The tripartite motif (TRIM) proteins form one of the largest subfamilies of RING-type E3 ubiquitin ligases, comprising more than 80 members. TRIM family members typically contain a RING domain usually catalyzing ubiquitin transfer; one or two B-box domains mediating protein–protein interactions; and a large coiled-coil domain region, which is involved in self-association or oligomerization with other TRIM E3-ligase proteins (Fiorentini et al., 2020, Ozato et al., 2008). About two-thirds of human TRIM proteins feature a PRYSPRY domain, also known as the B30.2 domain, in their C-terminal region. All characterized family members shared the same overall PRYSPRY twisted β-sandwich fold consisting of a 7-stranded and a 6-stranded antiparallel β-sheet.

Conversely, the TRIM36 PRYSPRY domain has characteristic loop insertions, which also affects its oligomerization state. The crystal lattice of the TRIM36 PRYSPRY domain contained four molecules in the asymmetric unit, forming two essentially identical symmetrical dimers. This observation is consistent with the TRIM36 domain eluting in gel filtration with a Superdex-75 column at a retention time corresponding to a dimer. The dimer interface is formed by a helix-turn-strand insertion between the canonical β-strands 2 and 3 of the PRY subdomain. The additional β-strand, β2′, self-assembled into a two-stranded antiparallel intermolecular β-sheet, and Phe543, Leu545, Leu547, and Ile552, located on the helix, form hydrophobic packing interactions with the adjacent monomer. The total dimer interface area is 1803 Å2 for chains A and B, and 1875 Å2 for chains C and D. The same PRYSPRY dimer interface was also predicted in the AlphaFold3 model of the full-length protein of TRIM36, and the related TRIM46 homolog, in addition to the typical dimerization via the coiled-coil domain. An unusually large insertion was observed between the canonical β-strands 5 and 6, featuring an additional helix and a long disordered segment. Another noteworthy feature of the TRIM36 structure is a unique helical extension at the C-terminus. A systematic analysis of this canonical substrate-binding region in the PRYSPRY structures determined in this study revealed significant variations and distinct surface properties across different family members, providing intriguing insights into the divergent evolution of TRIM family members. This canonical binding site was accessible to a varying degree in the domains crystallized here, except for TRIM36. In this case, dimerization via the insertion between the canonical β-strands 2 and 3 effectively occluded much of the putative substrate-binding site.

>MTPPAPVFSFLFDEKCGYNNEHLLLNLKRDRVESRAGFNLLLAAERIQVGYYTSLDYIIGDTGITKGKHFWAFRVEPYSYLVKVGVASSDKLQEWLRSPRDAVSPRYEQDSGHDSGSEDACFDSSQPFTLVTIGMQKFFIPKSPTSSNEPENRVLPMPTSIGIFLDCDKGKVNFYDMDQMKCLYERQVDCSHTLYPAFALMGSGGIQLEEPITAKYLEYQEDMAENLYFQ[4x]> MEINPYLMFLNNDVTSLISTTYPYTGPPPMSHGSSTKYTLETIKRTYDYSRTSVEKTSKVFNIPRRKFCNCLEDKDELVKPTGNVDISSLLGLAEMMEKRMGEGFFKHCVMEAETEILKMHFSRLTEGRQTYDWTSERNMPAATALQLTVDAIKETEGPFKGTTMLEYCNKMIEMLDWKEIKFKKVKTVVRREKDKRSGKEIKTKVPVMGIDSIKHDEFLIRALTINTMAKDGERGKLQRRAIATPGMIVRPFSKIVETVAQKICEKLKESGLPVGGNEKKAKLKTTVTSLNARMNSDQFAVNITGDNSKWNECQQPEAYLALLAYITKDSSDLMKDLCSVAPVLFCNKFVKLGQGIRLSNKRKTKEVIIKAEKMGKYKNLMREEYKNLFEPLEKYIQKDVCFLPGGMLMGMFNMLSTVLGVSTLCYMDEELKAKGCFWTGLQSSDDFVLFAVASNWSNIHWTIRRFNAVCKLIGINMSLEKSYGSLPELFEFTSMFFDGEFVSNLAMELP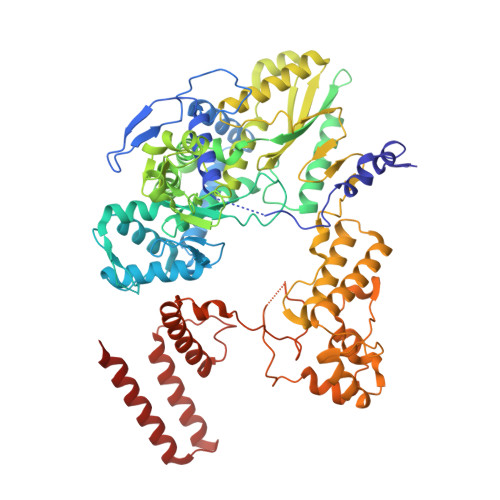AFTTAGVNEGVDFTAAMSIIKTNMINNSLSPSTALMALRICLQEFRATYRVHPWDSRVKGGRMKIINEFIKTIENKDGLLIADGGKLMNNISTLHIPEEVLKFEKMDEQYRNRVFNPKNPFTNFDKTIDIFRAHGPIRVEENEAVVSTHSFRTRANRTLLNTDMRAMMAEEKRYQMVCDMFKSVFESADINPPIGAMSIGEAIEEKLLERAKMKRDIGAIEDSEYEEIKDIIRDAKKARLESR> SMQVERESISRLMQNYEKINVNEITRFSDFPLSKKTLKGLQEAQYRLVTEIQKQTIGLALQGKDVLGAAKTGS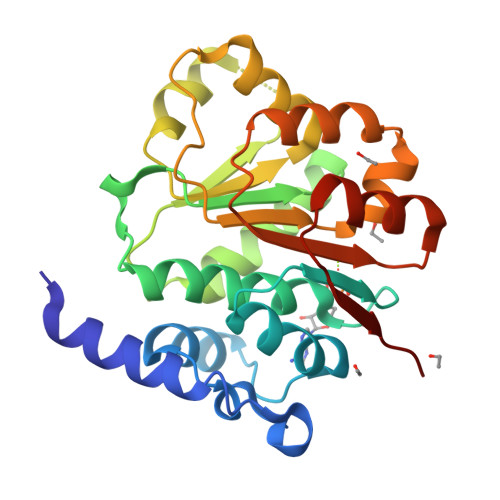GKTLAFLVPVLEALYRLQWTSTDGLGVLIISPTRELAYQTFEVLRKVGKNHDFSAGLIIGGKDLKHEAERINNINILVCTPGRLLQHMDETVSFHATDLQMLVLDEADRILDMGFADTMNAVIENLPKKRQTLLFSATQTKSVKDLARLSLKNPEYVWVHEKA>MSFEGKIALVTGASRGIGRAIAELLVERGACVIGTATSEKGAEAISAYLGENGKGLMLNVVDPTSIDTVLATIRAEFGEVDILVNNAGITRDNLLMRMKDDEWQDIIDTNLTSVFRLSKAVMRAMMKKRFGRIITIGSVVGTMGNAGQVNYAAAKAGVIGFSKSLAREVASRGITVNVV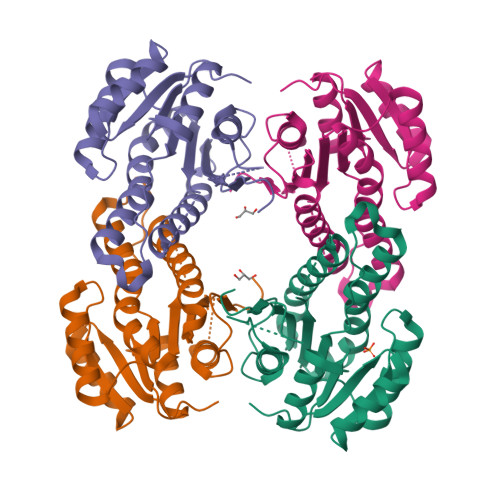APGFIETDMTRTLTDDQRAGILAQVPANRLGDAKEIASAVAFLASDEASYISGETLHVNGGMYMI[4x]> MGTGYYDDDAHGHVEADAAPRATTGTGTGSASQTVTIPCHHIRLGDILILQGRPCQVIRISTSAATGQHRYLGVDLFTKQLHEESSFVSNPAPSVVVQTMLGPVFKQYRVLDMQDGSIVAMTET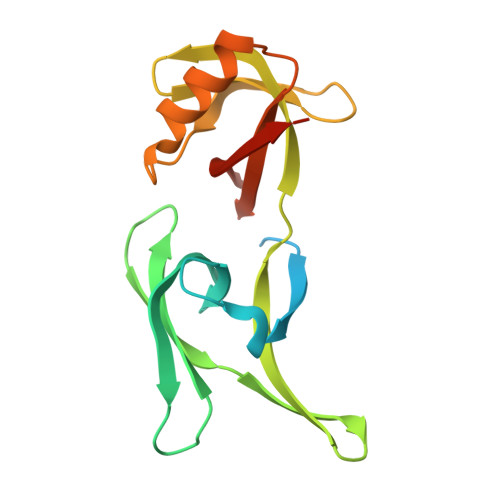GDVKQNLPVIDQSSLWNRLQKAFESGRGSVRVLVVSDHGREMAVDMKVVHGSRLAS(2,2-DIPHOSPHONOETHYL)(DODECYL)DIMETHYLPHOSPHONIUM 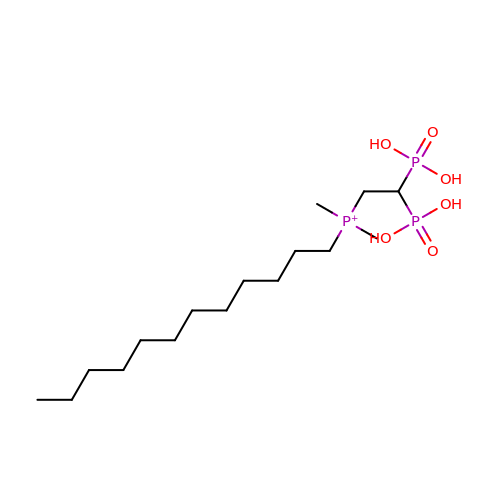| C16 H38 O6 P3 | QCMHKGWUOSRYCF-UHFFFAOYSA-O> KPKLLNKFDKTIKAELDAAEKLRKRGKIEEAVNAFKELVRKYPQSPRARYGKAQCEDDLAEKRRSNEVLRGAIETYQEVASLPDVPAD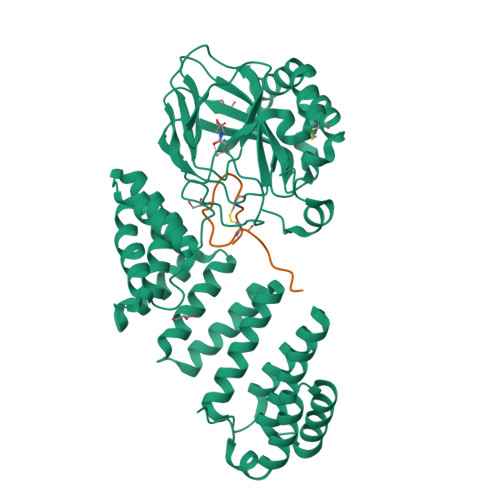LLKLSLKRRSDRQQFLGHMRGSLLTLQRLVQLFPNDTSLKNDLGVGYLLIGDNDNAKKVYEEVLSVTPNDGFAKVHYGFILKAQNKIAESIPYLKEGIESGDPGTDDGRFYFHLGDAMQRVGNKEAYKWYELGHKRGHFASVWQRSLYNVNGLKAQPWWTPKETGYTELVKSLERNWKLIRDEGLAVMDKAKGLFLPEDENLREKGDWSQFTLWQQGRRNENACKGAPKTCTLLEKFPETTGCRRGQIKYSIMHPGTHVWPATGPTNCRLRMHLGLVIPKEGCKIRCANETKTWEEGKVLIFDDSFEHEVWQDASSFRLIFIVDVWHPELTPQQRRSLPAI;> DGDQSETSPSQNQGKCKDGLGEYTCTSLEGFEGKNSELF N-[(2S,3R)-2-{[(1R,2S,3S,4R,6S)-6-amino-3-{[3-deoxy-4-C-methyl-3-(methylamino)-beta-L-lyxopyranosyl]oxy}-4-(ethylamino)-2-hydroxycyclohexyl]oxy}-6-(aminomethyl)-3,4-dihydro-2H-pyran-3-yl]acetamide 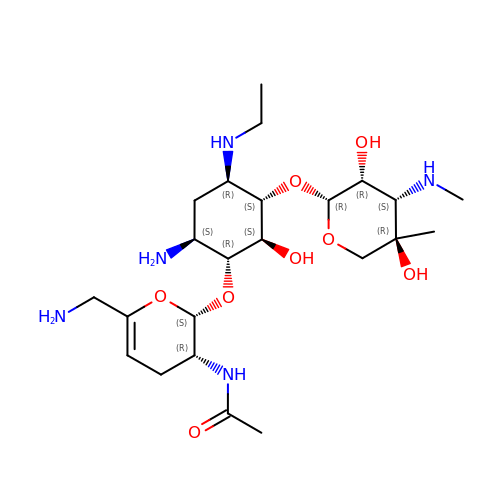| C23 H43 N5 O8 | GQIIPKQUZXGMPH-PWAQZHRDSA-N>[4x]GLVNFGNTCYCNSVLQALYFCRPFREKVLAYKSQPRKKESLLTCLADLFHSIATQKKKVGVIPPKKFITRLRKENELFDNYMQQDAHEFLNYLLNTIADILQEERKQEKQNGRLPNGNIDNENNNSTPDPTWVHEIFQGTLTNETRCLTCETISSKDEDFLDLSVDVEQNTSITHCLRGFSNTETLCSEYKYYCEECRSKQEAHKRMKVKKLPMILALHLKRFKYMDQLHRYTKLSYRVVFPLELRLFNTSGDATNPDRMYDLVAVVVHCGSGPNRGHYIAIVKSHDFWLLFDDDIVEKIDAQAIEEFYGLTSDISKNSESGYILFYQSRD;>[4x]MAAHHRQNTAGRRKVQVSYVIRDEVEKYNRNGVNALQLDPALNRLFTAGRDSIIRIWSVNQHKQDPYIASMEHH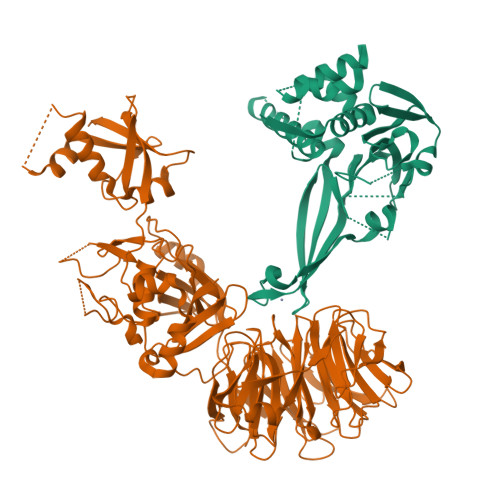TDWVNDIVLCCNGKTLISASSDTTVKVWNAHKGFCMSTLRTHKDYVKALAYAKDKELVASAGLDRQIFLWDVNTLTALTASNNTVTTSSLSGNKDSIYSLAMNQLGTIIVSGSTEKVLRVWDPRTCAKLMKLKGHTDNVKALLLNRDGTQCLSGSSDGTIRLWSLGQQRCIATYRVHDEGVWALQVNDAFTHVYSGGRDRKIYCTDLRNPDIRVLICEEKAPVLKMELDRSADPPPAIWVATTKSTVNKWTLKGIHNFRASGDYDNDCTNPITPLCTQPDQVIKGGASIIQCHILNDKRHILTKDTNNNVAYWDVLKACKVEDLGKVDFEDEIKKRFKMVYVPNWFSVDLKTGMLTITLDESDCFAAWVSAKDAGFSSPDGSDPKLNLGGLLLQALLEYWPRTHVNPMDEEENEVNHVNGEQENRVQKGNGYFQVPPHTPVIFGEAGGRTLFRLLCRDSGGETESMLLNETVPQWVIDITVDKNMPKFNKIPFYLQPHASSGAKTLKKDRLSASDMLQVRKVMEHVYEKIINLDNESQTTSSSNNEKPGEQEKEEDIAVLAEEKIELLCQDQVLDPNMDLRTVKHFIWKSGGDLTLHYRQKST> MNFNVSLMEKLKWKIKCIENKFLNYRLTTNETVVAETEYGKVKGVKRLTVYDDSYYSFEGIPYAQPPVGELRFKAPQRPTPWDGVRDCCNHKDKSVQVDFIAGKVCGSEDCLYLSVYTNNLNPETKRPVLVYIHGGDFIIGENHRDMYGPDYFIKKDVVLINIQYRLGALGFLSLNSEDLNVPGNAGLKDQVMALRWIKNNCANFGGNPDNITVFGESAGAASTHYMMLTEQTRGLFHRGILMSGNAICPWASTQCQHRAFTLAKLAGYKGEDNDKDVLEFLMKAKPQDLIKLEEKVLTLEERTNMVVFPFGPTVEPYQTADCVLPKHPREMVKTAWGNSIPTMMGNTSYEGLFFTSILKQTPMLVKELETCVNFVPSELADAERTAPETLEMGAKIKKAHVTGETPTADNFMDLCSHIYFWFPMHRLLQLRFNHTSGTPVYLYRFDFDSEDLINPWRIMRSGRGVKGVGHADELTYFFWNQLAKRM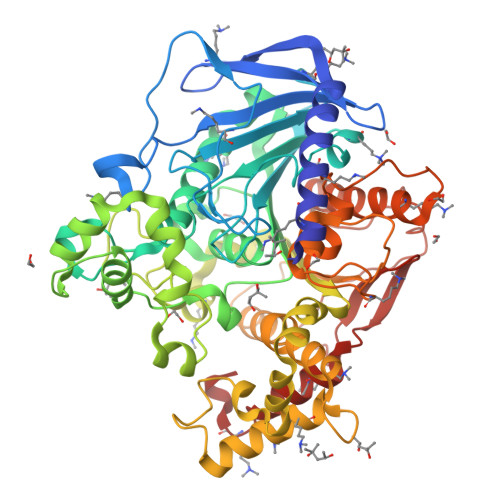PKESREYKTIERMTGIWIQFATTGNPYSNEIEGMENVSWDPVEKSDEVYRCLNISDELKMIDVPEMDKIKQWESMFEKHRDLF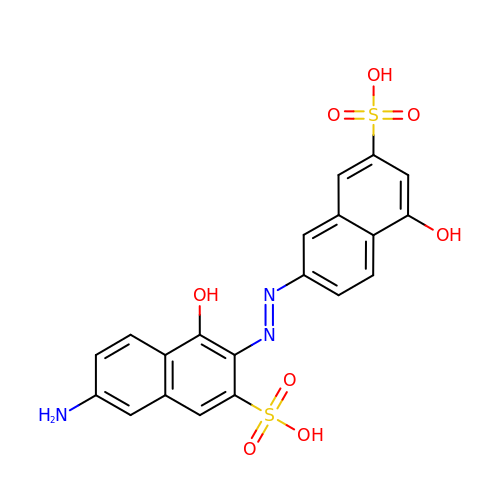7-amino-4-hydroxy-3-[(E)-(5-hydroxy-7-sulfonaphthalen-2-yl)diazenyl]naphthalene-2-sulfonic acid | C20 H15 N3 O8 S2 | ZSHNSNDVNDUHIM-GHVJWSGMSA-N>DMSHKEFTKFCYEVYNEIKISDKEFKEKRAALDTLRLCLKRISPDAELVAFGSLESGLALKNSDMDLCVLMDSRVQSDTIALQFYEELIAEGFEGKFLQRARIPIIKLTSDTKNGFGASFQCDIGFNNRLAI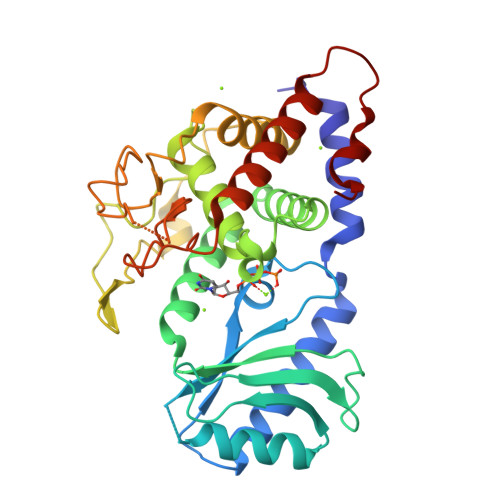HNTLLLSSYTKLDARLKPMVLLVKHWAKRKQINSPYFGTLSSYGYVLMVLYYLIHVIKPPVFPNLLLSPLKQEKIVDGFDVGFDDKLEDIPPSQNYSSLGSLLHGFFRFYAYKFEPREKVVTFRRPDGYLTKQEKGWTSATEHTGSADQIIKDRYILAIEDPFEISHNVGRTVSSSGLYRIRGEFMAASRLLNSRSYPIPYDSLFEEA[2x]>[4x]SNAMSTLGTLAPAADTELFADTLSCELRLPAGFHVTADPGSHATAETLLRSLGQVEDLRSEDSSEERGELPLLVQRMDAKLDLILALIGRLVRQSDTRLALGTVHWSVRGIRLASPHAHPPGTTGSVLLQPSDWLPELLQLPADVLASASDGQQHWLWLRFAPLGTGLQDALERHLFRLHRRQIADARRQR

Interestingly, after solving the XCC6012 crystal structure, we found that it adopts a novel quaternary PilZ variant that contains an intact PilZ-like domain, yet is interrupted in the middle by two long helices (α2 and α3). Four such XCC6012 molecules are intertwined into a stable tetramer via the heptad repeat α3 helices that form a parallel four-stranded coiled-coil. The quaternary structure of XCC6012 is found to adopt a novel “house-like” architecture, with a central pillar domain comprising the four vertical α3 helices, a roof-top domain comprising the eight inclined α2 and α4 helices, and four corner-stone domains comprising the PilZ domain. In contrast, the clipping treated with the xcc6012 knockout strain (XD62 #2 and XD62 #86) did not cause as much damage as that treated with the wild type strain. This experiment indicates that xcc6012 is indeed a pathogenic gene.

In brief, Se-Met substituted XCC6012 was found to form square-shaped crystals belonging to the space group P21, and contain four monomers and four acetate molecules per asymmetric unit. The final structure was obtained by repeated refinement to a resolution of 2.1 Å, with values of 22.0% and 24.6% for the Rcryst and Rfree, respectively. In addition, XCC6012 contains only a partial c-di-GMP binding signature motif (SxxG) and a long sequence of 57 amino acids comprising two α-helices (α2 and α3) after the β1 strand. But unlike other regular four-stranded coiled-coils, XCC6012 is further surrounded by four additional α2 and α4 helices, forming an intricate 12-helix bundle architecture. Three types of interactions are observed in this unique coiled-coil: Type I consisting of parallel α3 coiled-coil interactions (circled in red in Fig. 2); type II consisting of interconnected helix-helix (α2­α3) and helix-loop interactions (L6-α3, circled in blue Fig. 2), and type III consisting of α2-α4 helical interactions (circled in green in Fig. 2). The heptad repeat of the α3 helix contains purely the hydrophobic amino acids Val71, Leu78, Ile85 situating at position a, and Met74, Ile81, Leu88 at position d, respectively. In the surface of the coiled-coil, a pair of salt bridges between residue Lys77 at position g and residues Asp75 and Asp79 at position e and b, respectively, are observed, which stabilize the coiled-coil as are generally observed in other helix bundles. In addition, several hydrophobic residues are found to locate at positions c (Leu80), e (Leu82, Val89), or g (Leu84) that are normally occupied by hydrophilic residues and exposed to solvent. These altered hydrophobic residues are responsible for forming additional type II helical interactions. While wild type XCC6012 exhibited an unfolding temperature of 57.1°C, those of the K77D and D75K variants revealed unfolding temperature at 44.4C° and 53.9C°, which are substantially lower than those of the wild type by 12.7C° and 3.2C°, respectively.> GPGSSKHLNPGLQLYRASYEKNLPKMAEALAHGADVNWANSEENKATPLIQAVLGGSLVTCEFLLQ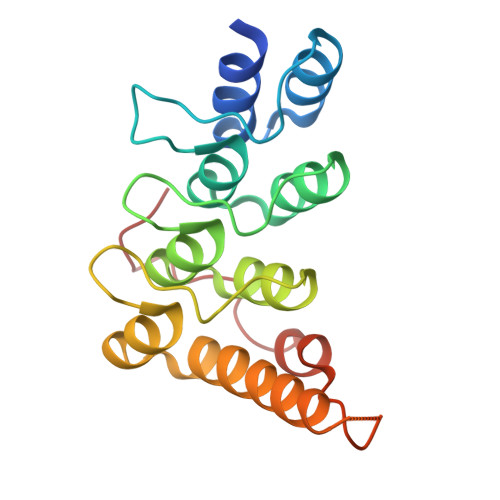NGANVNQRDVQGRGPLHHATVLGHTGQVCLFLKRGANQHATDEEGKDPLSIAVEAANADIVTLLRLARMNEEMRESEGLYGQPGDETYQDIFRDFSQMASNNPEKLNR> VPGPEYKVAILTVSDTVSAGAGPDRSGPRAVSVVDSSSEKLGGAKVVATAVVPDEVERIKDILQKWSDVDEMDLILTLGGTGFTPRDVTPEATKKVIERETPGLLFVMMQESLKITPFAMLA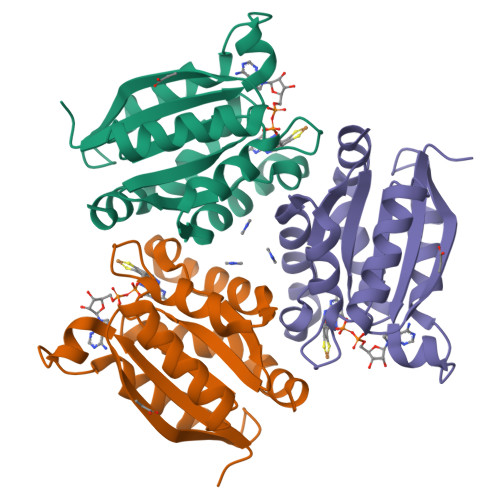RSAAGIRGSTLIINMPGNPNAVAECMEALLPALKHALKQIKGDKR>[2x]MNHKVHHHHHHIEGRHMTPSISKDAPIKGSITISKKGATFTAYKLLDAIKSGDAYEYSV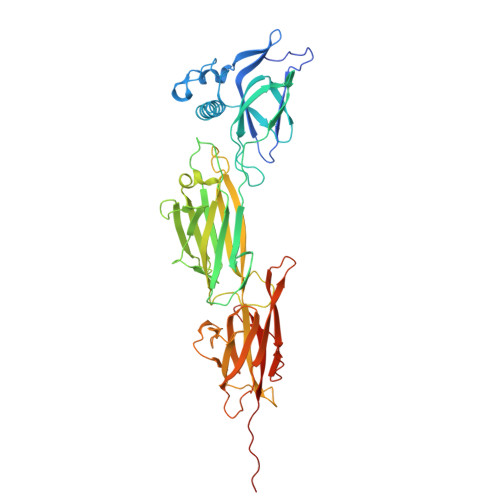NSDLKDFFNNSNYGSYSQESIQKLNGEQVKEFAINLHKYILENKKSGQELKDGQKNTVDLGYYLVTETSSDSEGAAVASTPIIVSVPQVSGDSWNYDVTINPKDNTPILEKNIVKENQRVKTSSENIGDVVKYEVKASIPVYQKNAQNIMYKFTDTMSKGLTYDEKTGFKVTSGDKVFAKDTDYTVDVKKQEDGSTVITINFVYENIKAYAETGITLNYQATLNKDAVISNKENLGNTNNIQLDYTNNPHVKDSYKKLTDKVTTYTFGFGITKVDSELNSKLLQGAEFSVKDAGGKIVAKYTYDEKGQVVYLSGNGVTNSKGITTFLGLKEGKYFITEEVAPSGYSLLKNPVEVTITANKDESGNYTGAATIEISNGNKAGQIINDISEKDGNILFNVQIENHAGFSLPSTGGLGNT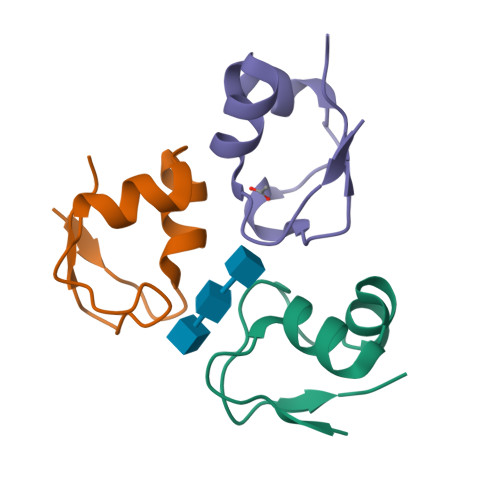>[3x]MYTVKPGDTMWKIAVKYQIGISEIIAANPQIKNPNLIYPGQKINIPNILEHHHHHH>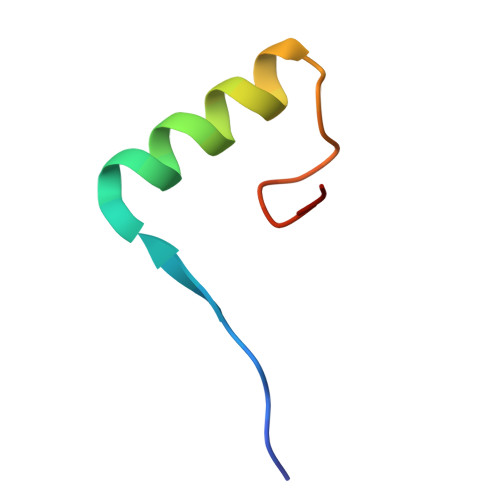 AAKVVYVFSTEMANKAAEAVLKGQVETIVSFHI>GSKPRGKMSSYAFFVQTCREEHKKKHPDASVNFSEFSKKCSERWKTMSAKEKGKFEDMAKADKA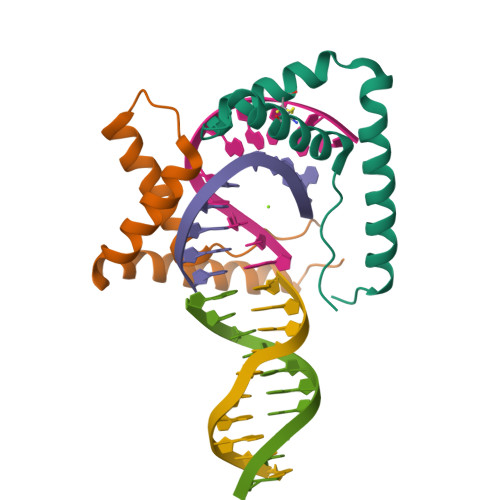RYEREMKTYIPP[2x]> AQSVPYGVSQIKAPALHSQGYTGSNVKVAVIDSGIDSSHPDLKVAGGASMVPSETNPFQDNNSHGTHVAGTVAALNNSIGVLGVAPSASLYAVKVLGADGSGQYSWIINGIEWAIANNMDVINMSLGGPSGSAALKAAVDKAVASGVVVVAAAGNEGTSGSSSTVGYPGKYPSVIAVGAVDSSNQRASFSSVGPELDVMAPGVSIQSTLPGNKYGAYNGTSMASPHVAGAAALILSKHPNWTNTQVRSSLENTTTKLGDSFYYGKGLINVQAAAQ;> YAPSALVLTVGKGVSATTAAPERAVTLTCAPGP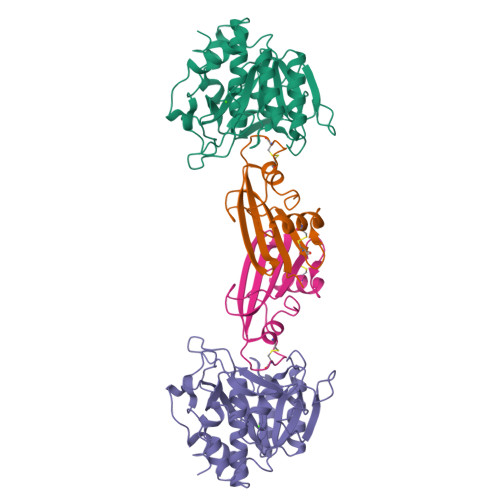SGTHPAAGSACADLAAVGGDLNALTRGEDVMCPMVYDPVLLTVDGVWQGKRVSYERVFSNECEMNAHGSSVFAF> SMTWLPLNPIPLKDRVSMIFLQYGQIDVIDGAFVLIDKTGIRTHIPVGSVACIMLEPGTRVSHAAVRLAAQVGTLLVWVGEAGVRVYASGQPGGARSDKLLYQAKLALDEDLRLKVVRKMFELRFGEPAP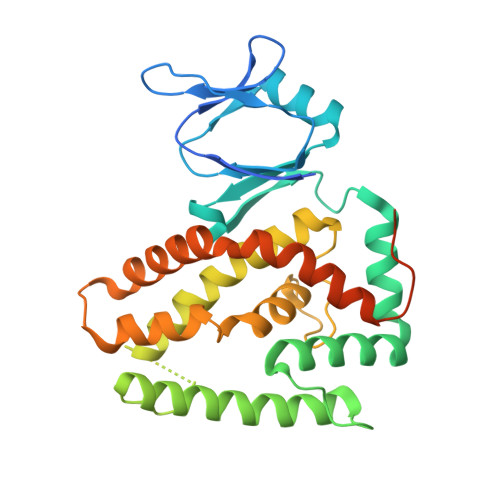ARRSVEQLRGIEGSRVRATYALLAKQYGVTWNGRRYDPKDWEKGDTINQCISAATSCLYGVTEAAILAAGYAPAIGFVHTGKPLSFVYDIADIIKFDTVVPKAFEIARRNPGEPDREVRLACRDIFRSSKTLAKLIPLIEDVLAAGEIQPPAPPEDAQPVAIPLPVSLGDAGHRSS> MTDNNKSSKTPNAWIAIDHNFSRAQVLTYYTLQLKGEHSLHQAISDNDWILVLDTTGNITRVGRILRIRSDLETTTIFFDRMLQVKSVVSIGITPFKFPPNDRAGRIQWTDFIETLPKELHITIADIPKIEDQTYIRELLQLAVMDDLLGPAGGPNELIVDMGVRDRYLVGKLAPREAAERGQEFPIDAEDIEDEEPDLIVKAKTAKVNSPSVLGSGETDTAEEIDAASNQSLVPSSLGMTFCVDGDVDRVEIEARWGRYERVPNDEHQFFKSNGQKAKVWKRIPCGGKIVLPLIEGSISHNAPDSTSPEVRVQGSIRAKNDNGDRLITLFLVNAQEEPDTNRDTAWVFQPELIVRAAKDAAKPAIFRRRPVLDADGMDPEREALEMIYRDRVEFAVGHGVAVHAEIADDVTLATEVRTTVMPQYEVQATETPGLELSDRPAMREMVSSGLLDMQRLATLDIDPLVDALSVLTNDYATWIDEQNLNVSSKAKGFDTQAQTAINRCQEIHTRLQEGINTLKSNENALAAFRFANQAMATQRIRSLYALAMRRGEDVTLDKFDVLKNRSWRPFQLAFLLLSIPSLADPCHPDRVKPIEAYADLLWFPTGGGKTEAYLGVAAFTMAIRRMQGNLGGYDSSRGLTVIMRYTLRLLTLQQFQRATALICAMEVLRREALNKGDKSLGTEPFTIGLWVGNKVTPGTTEDSHNAIEKTRNPGSYNAGTASPVQLTSCPWCGTEIVPGQDVEVKKDKAGGRTFVYCGDKKGRCEFSKGKSSTQPHPGIPVLVVDEEIYHRPPTMMIATVDKFAMMAWRGQVRTLFGRVEKECERHGLLWPGANCTGNHQAFKGQPSAKVKAIPPIRPPDLIIQDEFHLISGPLGTMVGLYETAVDELCSWTLNGKTVKPKIIASTATVRKAKEQVNNVFMRQVSVFPPHGLDVEDNFFSVQRHIKDKFGRRYLGVCSPGSSRPAMLIRVYTAFLTAAQELFDHFGEPADPYMTMVGYFNSLRELGGMKRLAEDDVQTRSYRVQMSMVERPALAQRSVNNIRELTSRVSSQDIPKYLDNLEVKFKAEFDSSAGKYVTKWQEGDTRAIDVVLATNMLSVGVDVNRLGLMAVNGQPKGTAEYIQATSRVGRSFPGLVCTVLTWARPRDLSHYETFEHYHATFYKHVEAQSVTPFSPRAMDRGLTGSLLSLMRLKNNEFSPNEGAGKLDMSNQSELAHAIEVLATRAGNVAEDNARKLLAENELKERADEWAKEASKGGRILGYEKRGPDKDKTVALIKSPGLQAWDNWTVPMSMREVESGVRLIMDTKFIKDDHDWKPRPATKDE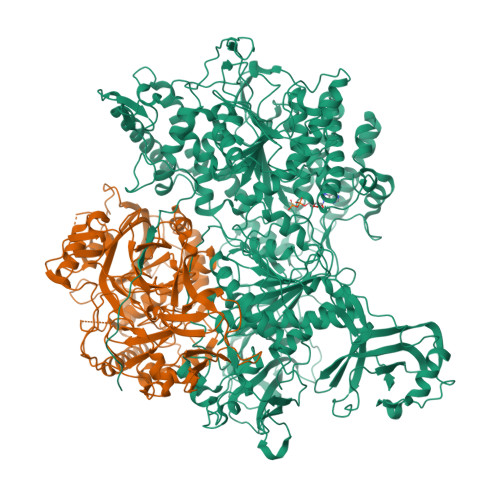D;> MIINNKTPVGEVRPSQLLWTYGPGALIDLPSLSVVTLGIDRWERERCQPIQEARLLAAVRKVLGPQVENLRMPPFQKSELVDPWSAEANIGVPVRPFPRWMRCVKCGLLSPFDDGLLEIKEDRFRAERTRFVHKGCTGSKGNLPAKDADAVPARFLLACRDGHLDDFPWHYFVHGGNSTCKGTLRFFESGASLQTENLWVRCDSCEASRSMAHAFGKAGKENLPACRGRHPHLDQFDIDCGEEPRAVLLGATNSWFPITLSALAIPQSKNPLSQLIQDGWPLFEAITAEVMVPIVVQTLKLTGGLPGIDKYSVSDIWSAIEMHRSGGDSEFVGEADIKGPEWEVLTEANPPTDYPHFMSKKIGTPAQFIPYISRVLLLERLREVNALLGFTRVEAPEGSGEINERPQMASLARNKPEWVPANQVHGEGIFIQFNEKTLVAWESLDAVKQVDEMLRGGHTGWRNSRNLDPNEDYPGIRYAMLHTLSHLLIRELALECGYNAASIRERIYADTSNGSPQAGILIYTAAADSDGTLGGLVDLGKPENLGRLLVQALNRSKICSSDPLCSEHNPEKDRSLHAAACHACTLVAETSCEQGNRYLDRSLLIPTLERIHAAFFKGF The structure of the eukaryotic chromosomal replicase, DNA polymerase (Pol) δ, was determined in complex with its cognate proliferating cell nuclear antigen (PCNA) sliding clamp on primed DNA. Pol δ performs lagging strand synthesis by extending primers generated by Pol α primase every 100 to 200 nt. In fact, Pol δ has little activity in the absence of PCNA, which stimulates Pol δ activity by a factor of 30 (16). Pol3 harbors the catalytic Pol and proofreading 3′-5′ exonuclease, and the regulatory subunits are Pol31 (i.e., the B subunit) and Pol32.

We introduced two mutations, D321S and E323S, into the proofreading 3′-5′ exonuclease active site of Pol3 to prevent degradation of the T/P DNA. The yeast Pol δ-PCNA-DNA-ddTTP structure is frozen at a stage at which the incoming ddTTP forms a Watson–Crick base pair with the template strand but is not incorporated into the primer because the last primer nucleotide is the dideoxyribonucleotide ddG. There are three conserved acidic residues (D608, D762, and D764) in the palm domain, two of which coordinate the two Mg2+ ions (residues D608 and D764) that in turn interact with the phosphodiester bonds of the incoming ddTTP. The structure shows that Pol3 is the only subunit of Pol δ that binds PCNA, mediated through a single subunit of the PCNA trimer. Surprisingly, Pol3 is the only subunit of Pol δ that binds PCNA, using a nonconsensus PIP site that binds only one PCNA protomer of the trimeric ring. The CysA element contains a nonconsensus PIP motif (997-GGLMSFI-1003) that is substantially distinct from the consensus PIP motif, as well as a zinc finger motif (amino acids 1,009 to 1,030) with its four cysteine residues (C1009, C1012, C1024, and C1027) coordinating the zinc ion (Zn2+). Interestingly, the regulatory subunits, Pol31 and Pol32, are oriented laterally with respect to the Pol3-PCNA-DNA axis and do not interact with DNA. Importantly, the 4Fe-4S cluster is centrally located in the holoenzyme and functions to glue together the Pol3 and the regulatory Pol31 and Pol32 subunits by interacting with the OB and PDE elements of Pol31, resulting in an extensive interface of 2,360 Å2. The EM map of Pol δ-PCNA-DNA shows 22 bp of ordered dsDNA extending from the Pol3 active site and through PCNA. Most interestingly, in the presence of Pol δ, the DNA is held at a nearly perpendicular angle (84°) to the plane of PCNA, and there appears to be no distortion of the B-form DNA.

> MSEKRSLPMVDVKIDDEDTPQLEKKIKRQSIDHGVGSEPVSTIEIIPSDSFRKYNSQGFKAKDTDLMGTQLESTFEQELSQMEHDMADQEEHDLSSFERKKLPTDFDPSLYDISFQQIDAEQSVLNGIKDENTSTVVRFFGVTSEGHSVLCNVTGFKNYLYVPAPNSSDANDQEQINKFVHYLNETFDHAIDSIEVVSKQSIWGYSGDTKLPFWKIYVTYPHMVNKLRTAFERGHLSFNSWFSNGTTTYDNIAYTLRLMVDCGIVGMSWITLPKGKYSMIEPNNRVSSCQLEVSINYRNLIAHPAEGDWSHTAPLRIMSFSISCAGRIGVFPEPEYDPVIQIANVVSIAGAKKPFIRNVFTLNTCSPITGSMIFSHATEEEMLSNWRNFIIKVDPDVIIGYNTTNFDIPYLLNRAKALKVNDFPYFGRLKTVKQEIKESVFSSKAYGTRETKNVNIDGRLQLDLLQFIQREYKLRSYTLNAVSAHFLGEQKEDVHYSIISDLQNGDSETRRRLAVYCLKDAYLPLRLMEKLMALVNYTEMARVTGVPFSYLLARGQQIKVVSQLFRKCLEIDTVIPNMQSQASDDQYEGATVIEPIRGYYDVPIATLDFNSLYPSIMMAHNLCYTTLCNKATVERLNLKIDEDYVITPNGDYFVTTKRRRGILPIILDELISARKRAKKDLRDEKDPFKRDVLNGRQLALKISANSVYGFTGATVGKLPCLAISSSVTAYGRTMILKTKTAVQEKYCIKNGYKHDAVVVYGDTDSVMVKFGTTDLKEAMDLGTEAAKYVSTLFKHPINLEFEKAYFPYLLINKKRYAGLFWTNPDKFDKLDQKGLASVRRDSCSLVSIVMNKVLKKILIERNVDGALAFVRETINDILHNRVDISKLIISKTLAPNYTNPQPHAVLAERMKRREGVGPNVGDRVDYVIIGGNDKLYNRAEDPLFVLENNIQVDSRYYLTNQLQNPIISIVAPIIGDKQANGMFVVKSIKINTGSQKGGLMSFIKKVEACKSCKGPLRKGEGPLCSNCLARSGELYIKALYDVRDLEEKYSRLWTQCQRCAGNLHSEVLCSNKNCDIFYMRVKVKKELQEKVEQLSKW;> MDALLTKFNEDRSLQDENLSQPRTRVRIVDDNLYNKSNPFQLCYKKRDYGSQYYHIYQYRLKTFRERVLKECDKRWDAGFTLNGQLVLKKDKVLDIQGNQPCWCVGSIYCEMKYKPNVLDEVINDTYGAPDLTKSYTDKEGGSDEIMLEDESGRVLLVGDFIRSTPFITGVVVGILGMEAEAGTFQVLDICYPTPLPQNPFPAPIATCPTRGKIALVSGLNLNNTSPDRLLRLEILREFLMGRINNKIDDISLIGRLLICGNSVDFDIKSVNKDELMISLTEFSKFLHNILPSISVDIMPGTNDPSDKSLPQQPFHKSLFDKSLESYFNGSNKEILNLVTNPYEFSYNGVDVLAVSGKNINDICKYVIPSNDNGESENKVEEGESNDFKDDIEHRLDLMECTMKWQNIAPTAPDTLWCYPYTDKDPFVLDKWPHVYIVANQPYFGTRVVEIGGKNIKIISVPEFSSTGMIILLDLETLEAETVKIDI;> MDQKASYFINEKLFTEVKPVLFTDLIHHLKIGPSMAKKLMFDYYKQTTNAKYNCVVICCYKDQTIKIIHDLSNIPQQDSIIDCFIYAFNPMDSFIPYYDIIDQKDCLTIKNSYELKVSESSKIIERTKTLEEKSKPLVRPTARSKTTPEETTGRKSKSKDMGLRSTALLAKMKKDRDDKETSRQNELRKRKEENLQKINKQNPEREAQMKELNNLFVEDDLDTEEVNGGSKPNSPKETDSNDKDKNNDDLEDLLETTAEDSLMDVPKIQQTKPSETEHSKEPKSEEEPSSFIDEDGYIVTKRPATSTPPRKPSPVVKRALSSSKKQETPSSNKRLKKQGTLESFFKRKAK;>MLEAKFEEASLFKRIIDGFKDCVQLVNFQCKEDGIIAQAVDDSRVLLVSLEIGVEAFQEYRCDHPVTLGMDLTSLSKILRCGNNTDTLTLIADNTPDSIILLFEDTKKDRIAEYSLKLMDIDADFLKIEELQYDSTLSLPSSEFSKIVRDLSQLSDSINIMITKETIKFVADGDIGSGSVIIKPFVDMEHPETSIKLEMDQPVDLTFGAKYLLDIIKGSSLSDRVGIRLSSEAPALFQFDLKSGFLQFFLAPKFNDEE[3x]> GTTKHSKLLILGSGPAGYTAAVYAARANLQPVLITGMEKGGQLTTTTEVENWPGDPNDLTGPLLMERMHEHATKFETEIIFDHINKVDLQNRPFRLNGDNGEYTCDALIIATGASARYLGLPSEEAFKGRGVSASATCDGFFYRNQKVAVIGGGNTAVEEALYLSNIASEVHLIHRRDGFRAEKILIKRLMDKVENGNIILHTNRTLEEVTGDQMGVTGVRLRDTQNSDNIESLDVAGLFVAIGHSPNTAIFEGQLELENGYIKV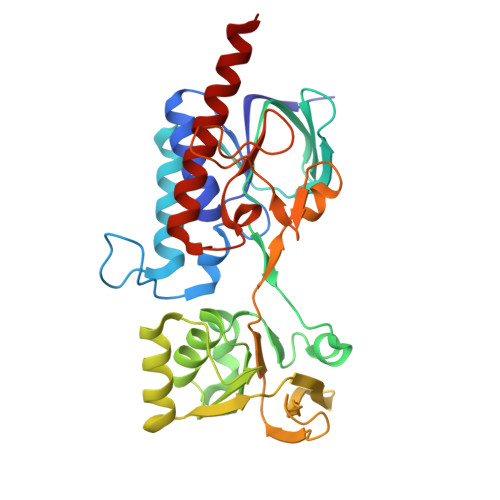QSGIHGNATQTSIPGVFAAGDVMDHIYRQAITSAGTGCMAALDAERYLDGLADAK> GHMSGEAPLTATVDGIIQPMLKAYRIPGMAVAVLKDGKAHYFNYGVANRESGQRVSEQTLFEIGSVSKTLTATLGAYAAVKGGFELDDKVSQHAPWLKGSAFDGVTMAELATYSAGGLPLQFPDEVDSNDKMQTYYRSWSPVYPAGTHRQYSNPSIGLFGHLAANSLGQPFEQLMSQTLLPKLGLHHTYIQVPESAMANYAYGYSKEDKPIRATPGVLAAEAYGIKTGSADLLKFVEANMGYQGDAALKSAIALTHTGFH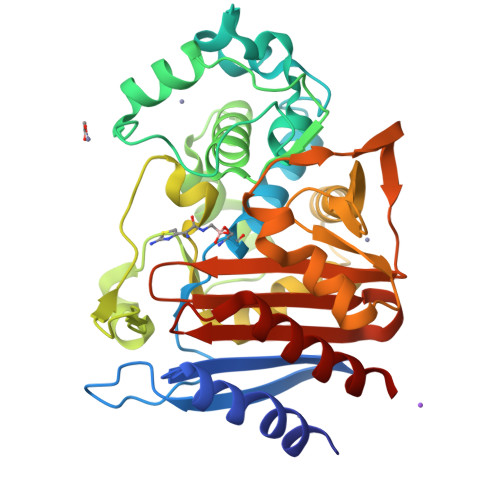SVGEMTQGLGWESYDYPVTEQVLLAGNSPAVSFQANPVTRFAVPKAMGEQRLYNKTGSTGGFGAYVAFVPARGIAIVMLANRNYPIEARVKAAHAILSQLAE>[2x]MGSSHHHHHHSQDPMTVTANQVLRPRGPQIERLTDNRAKVVIEPLERGYGHTLGNALRRVLLSSIPGFAITEVEIDGVLHEYTTVEGLQEDVLDVLLNLKDVAIRMHSGDSATLSLSKQGPGTVTAADIRTDHNVEIINGDHVICHLTKDTALNMRLKIERGFGYQPAAARRRPDEETRTIGRLMLDASFSPVRRVAYAVEAARVEQRTDLDKLVIDIETNGTIDAEEAVRTAADILSDQLSVFGDFTHRDRGAAKPAASGVDPVLLRPIDDLELTVRSANCLKAESIYYIGDLIQKTEVELLKTPNLGKKSLTEIKEVLAQRGLALGMKLENWPPAGVAQHGMLG;> MTSYSFTEKKRIRKDFGKQRSILEVPFLLAIQVDSYREFLQEDVESTKRKDLGLHAALKSVFPISSYSGNAALEYVGYKLGQPVFDERECRQRGMSYGAPLRVTVRLVIYDRESSTKAIKYVKEQEVYLGEIPLMTGNGTFIVNGTERVIVSQLHRSPGVFFDHDRGKTHSSGKLLYSARIIPYRGSWLDFEFDPKDALFTRIDRRRKLPVSILLRALGYNNEEMLAEFFEINTFHINPDEGVQLELVPERLRGETLNFDLADGDKVIVEAGKRITARHVKQLEAAGVAALAVPDDYLVGRILSHDVVDGSTGELLANANDEISEDQLTAFRKAGVDAVGTLWVNDLDRGPYLSNTLRIDPTKTQLEALVEIYRMMRPGEPPTKEAAQNLFHNLFFTFERYDLSTVGRMKFNRRVGRKDVLGESVLYDKKYFAERNDEESKRLVAEHTDTSDILEVIKVLTEIRNGRGVVDDIDHLGNRRVRSVGEMAENVFRVGLVRVERAVKERLSMAESEGLTPQELINAKPVAAAIKEFFGSSQLSQFMDQNNPLSEVTHKRRVSALGPGGLTRERAGFEVRDVHPTHYGRVCTIETPEGPNIGLINSLAVFARTNQYGFLETPYRKVLDGKVSDDVEYLSAIEENEYVIAQANALTDAKNMLTEQFVPCRFQGESLLKPPSEVHFMDVSPMQTVSVAAALVPFLEHDDANRALMGANMQRQAVPTLRSQKPLVGTGIERAVARDSGVTVNALRGGVIEQIDAARIVVKVNEAEIGGGTDAGVDIYNLIKYTRSNQNTCINQRPLVNVGDVIARGDVLADGPSTDIGELALGQNMLIAFMPWNGYNFEDSILLSERVVEEDRYTTIHIEELTCVARDTKLGPEEISADIPNVSEQALNRLDESGVVYIGAEVRAGDIMVGKVTPKGESQLTPEEKLLRAIFGEKASDVKDSSLRVPPGMDGTVIDVQVFTRDGIEKDKRARQIEENEIKRVKKDFDDQFRILEAAIYARLRSQIVGKVANGGANLKKGDSVTDAYLDGLKKSDWFQLRMKDEDAADAIERAQKQIQAHEKEFEARFADKRGKITQGDDLAPGVLKMVKVFLAVKRRIQPGDKMAGRHGNKGVVSNVVPVEDMPYMATGESVDIVLNPLGVPSRMNIGQILEVHLGWAAKGLGRKIQRMLEAQAAVSELRKFLDDIYNHDNAINAQRVDLSQFSDEELLNLGKNLIDGVPMATPVFDGASEAEIKRMLELADLPQSGQTQLYDGRTGEAFDRKTTVGYMHYLKLNHLVDDKMHARSTGPYSLVTQQPLGGKAQFGGQRFGEMEVWALEAYGAAYTLQEMLTVKSDDVQGRNQMYKNIVDGEHEMVAGMPESFNVLVKEIRSLAIHMELEE;> MKDLLNLFNQQRQTLDFDAIKIALASPDLIRSWSYGEVKKPETINYRTFKPERDGLFCAAIFGPIKDYECLCGKYKRMKHRGVVCEKCGTEVTLAKVRRERMGHIDLASPVAHIWFLKSLPSRIGLMLDMTLRDIERVLYFEAYVVTEPGLTPLERRQLLTEEQYLTARQEYNDDFDAAMGAEAVYELLRTIDLQSEMTRLREEIASTGSETKLKRLTKRIKLIEAFLESGNRPEWMVMTVLPVLPPDLRPLVPLDGGRFATSDLNDLYRRVINRNNRLRRLLELNAPDIIVRNEKRMLQESVDALLDNGRRGRAITGTNKRPLKSLADMIKGKQGRFRQNLLGKRVDYSGRSVITVGPYLKLHQCGLPKKMALELFKPFVFAKLQRRGLATTIKAAKKLVEREEAEVWDILEEVIREHPVLLNRAPTLHRLGIQAFEPVLIEGKAIQLHPLVCTAFNADFDGDQMAVHVPLSLEAQLEARALMMSTNNILSPANGEPIIVPSQDVVLGLYYMSRALENKKGEGMVFANTSEVKRAYDNRVVELHAKVKVRITQVDVDAVDGKRTSGTSIVDTTVGRALLSEILPEGLPFQLANTEMTKKNISRLINSSYRLLGLKDTVVFADKLMYTGYAYATRAGVSIGIDDMLIPDEKKGILTEAEAEVLEIQEQYQSGLVTAGERYNKVVDIWSRTSERIAKAMMDTIGTEKVENAKGETIDQKSMNSLYIMADSGARGSQAQIRQLAGMRGLMARPDGSIIETPIKANFREGLNVQEYFNSTHGARKGLADTALKTANSGYLTRRLVDVAQDVVITEIDCGTTEGLIMTPIVEGGDVVEPLKERVLGRVVAEDVYLPGNDEEPIVTRNTLLDEAWVAKLEDASVQSVKVRSTISCESSFGVCARCYGRDLARGHQVNIGEAVGVIAAQSIGEPGTQLTMRTFHIGGAASRAAAVDNITVKTTGSVKFNNLKSVAHASGSLVAVSRSGELSVLDGHGRERERYKLPYGATITAKDGDAVKAGQSVANWDPHNHPIVSEVAGFIRFIDFVDGVTVIEKTDELTGLASREITDPKRRGAHAKELRPIVRIVDGKGNDLTIPNTDLPAQYLLPPRSIVNLQDGAAVGVGDVVAKIPQEASKTRDITGGLPRVADLFEARKPKDPAILAERSGIISFGKDTKGKQRLIIKDTDGSEHEELIPKYRQIIVFEGEHVTKGETVVDGEPSPQDILRLLGVEPLAAYLVKEIQDVYRLQGVKINDKHIEVITRQMLRKVEIVDQGNSKFLNGEQVERQRVIEENARLVKRNELPAKYDPVLLGITKASLATESFISAASFQETTRVLTEAAVRGTRDNLRGLKENVIVGRLIPAGTGLAYHAGRRKASGLTDSEMETLSGKPAGAEPVAALADAGADEE;> MARITVEDCLEVVNNRFELVMMASKRARQLANGVQPLIENAAASDKPTVMALREIAARRIDNALIDEVEKAERERAEREALEWAAAEVVADEDMSKNDD;> GAMAMNEFTQISGYVNAFGSQRGSVLTVKVENDEGWTLVEEDFDRADYGSDPEFVAEVSSYLKRNGGIKDLTKVLTR

P7 is the key phage protein to regulate gene expression programs of both host bacteria and phage Xp10. P7 binds to host RNA polymerase to inhibit transcription of host genes. P7 turns on transcription of late genes of phage Xp10 by assisting host RNA polymerase in bypassing intrinsic terminators preceding the late genes. The structures reveal a unique binding site (the RNA-exit channel) of the phage protein P7 on bacterial host RNAP, where P7 exerts dual regulatory activities on host RNAP—inhibiting transcription initiation and preventing transcription termination.

In this study, we determined a cryo-EM structure of Xoo transcription elongation complex with P7 (P7-TEC) at 3.95 Å and a cryo-EM structure of Xoo transcription elongation complex with P7 and NusA (P7-NusA-TEC) at 3.41 Å. The overall structures of RNAP and the interactions between P7 and RNAP are essentially the same in the two structures. Our cryo-EM structures show that P7 almost completely blocks the RNA-exit channel. In the structures of P7-NusA-TEC and P7-TEC, such gate is largely blocked by P7 and leaves limited space for even a single-stranded RNA. The structure of P7-TEC graphically signifies that P7 inhibits intrinsic termination by preventing the second step—formation of the termination RNA hairpin. The other side of the β sheet approaches to but does not make interaction with the flap domain of RNAP-β subunit (βflap) in both P7-TEC and P7-NusA-TEC structures. The structure of P7-TEC also reveals an incompatible binding of P7 and domain 4 of σ70 (σ704) to RNAP. P7 makes interactions with the β′dock, β′ZBD, as well as βCTR, all of which are structural elements required for σ704 to anchor RNAP core enzyme. Furthermore, the flap-tip helix βFTH—the most important anchor point on RNAP for σ704—is displaced by P7 and becomes disordered in the structure of P7-TEC.>[2x]MAVTYEKTFEIEIINELSASVYNRVLNYVLNHELNKNDSQLLEVNLLNQLKLAKRVNLFDYSLEELQAVHEYWRSMNRYSKQVLNKEKVA;>MANIVNFTDKQFENRLNDNLEELIQGKKAVESPTAFLLG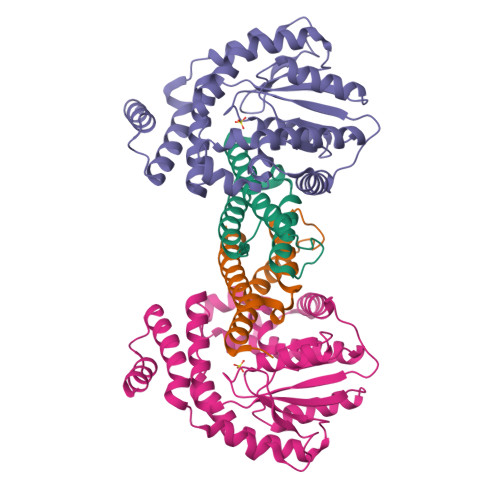GQPGSGKTSLRSAIFEETQGNVIVIDNDTFKQQHPNFDELVKLYEKDVVKHVTPYSNRMTEAIISRLSDQGYNLVIEGTGRTTDVPIQTATMLQAKGYETKMYVMAVPKINSYLGTIERYETMYADDPMTARATPKQAHDIVVKNLPTNLETLHKTGLFSDIRLYNREGVKLYSSLETPSISPKETLEKELNRKVSGKEIQPTLERIEQKMVLNKHQETPEFKAIQQKLESLQPPTPPIPKTPKLPGI[2x]> MHHHHHHVMIMKAFISENVRGIYAFDENGNLIEKRYFTDKPEKVLDQLLKGEITKDLEELLNSLKEKGYDEFVFEHPELSRRAKELGFSATTEFPNIAGERLRSNPEEFLGENWFEEYYKVGVALTRMRIQEQSGARDKMVIQAIEALDDINLLVARLREWYSLHFPELDELLPKHPQYVAFVKTVGHRDNINEEVLRELGLSEEKIKKILEAKEKTMGAWMDQTDIEVVRQLAEEIQLRKKLEDYIDRAMDDVAPNLKALVGAKLAARL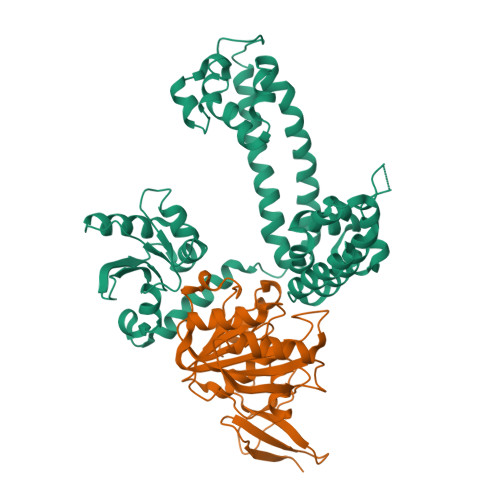ISLAGGLRELAMMPSSTIQVLGAEKALFRHLRTGAKPPKHGVIYQYPAINRSPWWQRGKIARALAGKLAIAARVDYFSGEYIAEELKKELEARIREIKEKY;> MHHHHHHMVEVKKHKFPGVYVVIDDDGSEKIATKNLVPGQRVYGERVIKWEGEEYRIWNPHRSKLGAAIVNGLKNFPIKPGKSVLYLGIASGTTASHVSDIVGWEGKIYGIEFSPRVLRELVPIVEERRNIIPILGDATKPEEYRALVTKVDVIFEDVAQPTQAKILIDNAKAYLKRGGYGMIAVKSRSIDVTKEPEQVFKEVERELSEYFEVIERLNLEPYEKDHALFVVRKP> MGSSHHHHHHSQDLMVTSTYIPMSQRRSWADVKPIMQDDGPNPVVPIMYSEEYKDAMDYFRAIAAKEEKSERALELTEIIVRMNPAHYTVWQYRFSLLTSLNKSLEDELRLMNEFAVQNLKSYQVWHHRLLLLDRISPQDPVSEIEYIHGSLLPDPKNYHTWAYLHWLYSHFSTLGRISEAQWGSELDWCNEMLRVDGRNNSAWGWRWYLRVSRPGAETSSRSLQDELIYILKSIHLIPHNVSAWNYLRGFLKHFSLPLVPILPAILPYTASKLNPDIETVEAFGFPMPSDPLPEDTPLPVPLALEYLADSFIEQNRVDDAAKVFEKLSSEYDQMRAGYWEFRRRECAE;> MATEFTPSVYSLVSKPLPSNSRPSATLDEQAETEDLISQLFDLTADPNALVSEHGKRYSGLRKQEHTQFLASSFFQLPGKFVSLDASRPWLVFWTVHSLDLLGVALDQGTKDRVVSTLLHFLSPKGGFGGGPANSQIPHLLPTYASVCSLAIAGNDSSTGGWKDLAAARQSIYEFFMRCKRPDGGFVVCEGGEVDVRGTYCLLVVATLLDIITPELL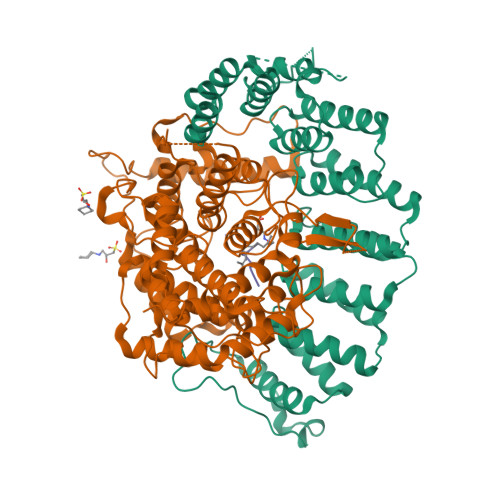HNVDKFVSACQTYEGGFACASFPFPSVVPSTSAFPTSEPSCRVSMAEAHGGYTSCSLNSHFLLTSVPLPSFPLSIDANAALRWTVLQQGEPIEGGGFRGRTNKLVDGCYSWWVGGGAPVAEELVRREKSRKVKKSRIEVFEEEKEGDWEDVPPIPPIFNRVALQEFTLVAAQQDPGSTGGLRDKPGKRPDQYHTCNNLSGLSIAQHKMSHSPSTVSSNRLKFDASKGLPAVKPVAPGGGWKNEDERQNARREIWANALGWIEEEGGEIIVGGKDNRINTTTPVFNILGLRLKPFINYFYCQEN;> TKCVVM>ASAAEQAAFRLVGHRNFVRFNPRSDRFHTLAFHHVELWCADAASAAGRFSFGLGAPLAARSDLSTGNSAHASLLLRSGSLSFLFTAPYAHGADAATAALPSFSAAAARRFAADHGLAVRAVALRVADAEDAFRASVAAGARPAFGPVDLGRGFRLAEVELYGDVVLRYVSYPDGAAGEPFLPGFEGVASPGAADYGLSRFDHIVGNVPELAPAAAYFAGFTGFHEFAEFTTEDVGTAESGLNSMVLANNSENVLLPLNEPVHGTKRRSQIQTFLDHHGGPGVQHMALASDDVLRTLREMQARSAMGGFEFMAPPTSDYYDGVRRRAGDVLTEAQIKECQELGV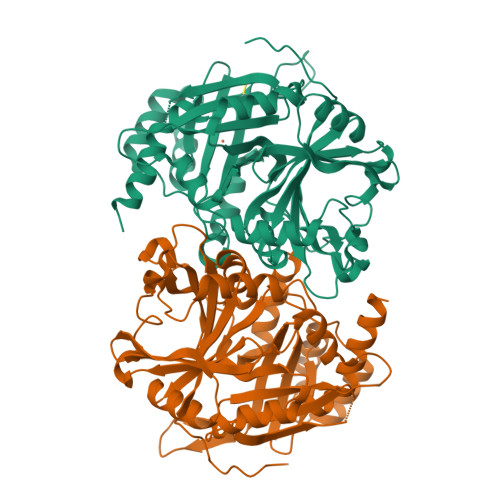LVDRDDQGVLLQIFTKPVGDRPTLFLEIIQRIGCMEKDEKGQEYQKGGCGGFGKGNFSQLFKSIEDYEKSLEAKQ[4x]>AVPETRPNHTIYINNLNEKIKKDELKKSLHAIFSRFGQILDILVSRSLKMRGQAFVIFKEVSSATNALRSMQGFPFYDKPMRIQYAKTDSDIIAKMK[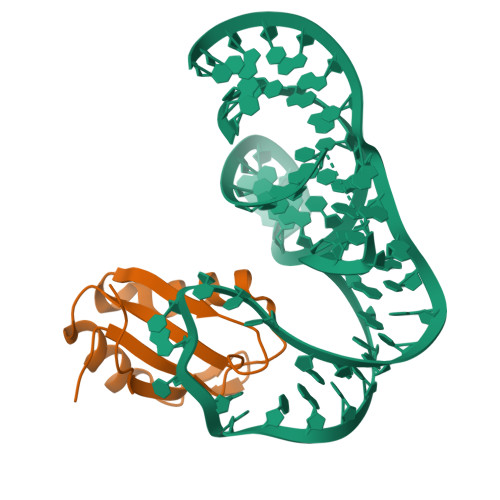2x]>SNAMSAVTYTFLGPQGTFTEAALMQVPGAADATRIPCTNVNTALERVRAGEADAAMVPIENSVEGGVTATLDAIATGQELRIIREALVPITFVLVARPGVELSDIKRISTHGHAWAQCRLWVDEHLPNADYVPGSSTAASAMGLLEDDAPYEAAICAPLIAAEQPGLNVLAEDIGDNPDAVTRFILVS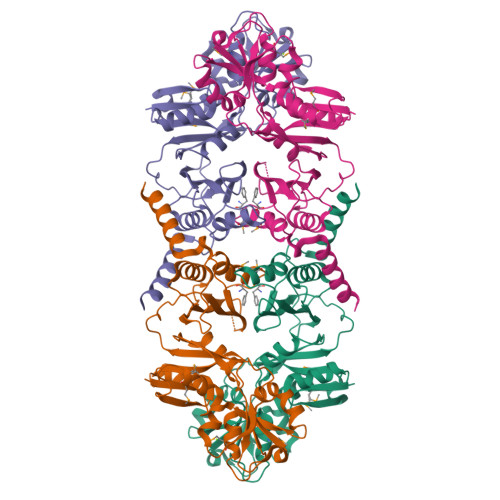RPGALPERTGADKTTVVVPLPEDHPGALMEILDQFASRGVNLSRIESRPTGQYLGHYFFSIDADGHATDSRVADALAGLHRISPATRFLGSYARADKQPAVVAPHTSDAAFASAHAWVDSILKGS[2x]> TPLVHVASVEKGRSYEDFQKVYNAIALKLREDDEADNYIGYGPVLVRLAWHTSGTWDKHDNTGGSYGGTYRFKKEFNDPSNAGLQNGFKFLEPIHKEFPWISSGDLFSLGGVTAVQEMQGPKIPWRCGRVDTPEDTTPDNGRLPDADKDADYVRTFFQRLNMNDREVVALMGAHALGKTHLKRSGYEGPFGAANNVFTNEFYLNLLNEDWKLEKNDANNEQWDSKSGYMMLPTDYSLIQDPKYLSIVKEYAN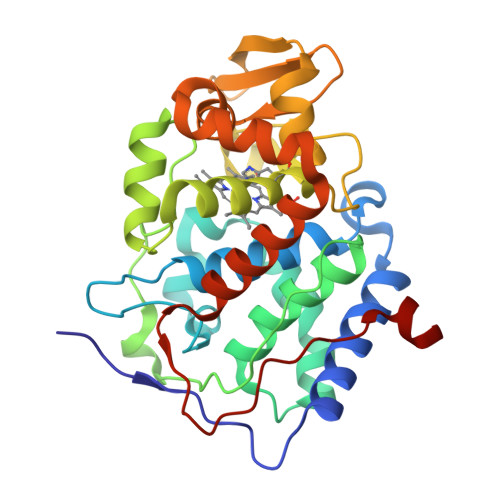DQDRFFKDFSKAFEKLLENGITFPKDAPSPFIFKTLEEQGL> MEAVLSRQAATAEAIGRFQDSSTSVGLVAGSPSTRIRRQADNVVLKSTSQAGDTLNDVIQDPTRRNKLINDNNLLKGIIMGRDGPVPSSRELIVRPDTLRAIINNRATIETTTMEAEFTETLMESNYNSASVKVSAPFITANSEYSESSSFKNTETEKSMYTSSRYLFPQGRIDFTTPDSGFDDVIKLSPQFTSGVQAALAKATGTEKREALQNLFQEYGHVFRTKVHIGGVLSAHTMETFSRSENETEVKQDVKAGLEGAVKGWGGGATAGHGNTQGTITTSQNRKLNVKYIVNGGDYTKIQNTEEWVASTNQSEHWRVIEVTEVTAVADLLPQPIRGQVKDLLKPLLGKWVDVEKVPGLESLPVSVYRPKGAIPAGWFWLGDTADASKALLVKPTLPARSGRNPALTSLHQGSGMTEQPFVDLPQYQYLSTYFGSFAHDTPPGSTLRGLRPDHVLPGRYEMHGDTISTAVYVTRPVDVPFPEDECFDLKSLVRVKLPGSGNPPKPRSALKKSMVLFDSGEK

To gain further insight into the structural conversions in pore formation, we chose pleurotolysin (Ply), a MACPF protein consisting of two components, PlyA and PlyB, from Pleurotus ostreatus. Previous studies have shown that PlyA binds membranes and is required to recruit the pore-forming MACPF protein PlyB to the membrane surface. PlyA and PlyB together form relatively small and regular pores in liposomes. The membrane attack complex/perforin-like family (MACPF) proteins form the largest superfamily of pore-forming proteins identified to date.

The 2.2 Å structure of PlyB reveals an N-terminal MACPF domain (blue/red/yellow) followed by three small β-rich domains clustered in a globular trefoil-like arrangement (green). The MACPF domain of PlyB contains a central, four-stranded bent and twisted β-sheet characteristic of the MACPF/CDC superfamily (red). The TMH1 cluster of helices (yellow) is located on the inside of PlyB, next to the concave face of the central β-sheet. TMH2 (yellow) comprises a single large α-helix and an additional β-strand (termed “strand β5”), located on the edge of the central β-sheet. Together, the central β-sheet and the TMH regions constitute the topologically conserved MACPF/CDC pore-forming fold. A single PlyB moiety was fitted into the upper part of the pore structure. The C-terminal trefoil (green) and the α-helices at the top of the MACPF domain (blue) unambiguously fit the EM density with only minor structural rearrangement.AASS is a bifunctional enzyme with an N-terminal lysine-2-oxoglutarate reductase (LOR) domain and a C-terminal saccharopine dehydrogenase (SDH) domain, which are homologous to Saccharomyces cerevisiae LYS1 and LYS9, respectively. The LOR domain catalyses the reductive deamination of L-lysine and 2-oxoglutarate into saccharopine (EC 1.5.1.8), which constitutes the first committed, and possibly rate-limiting, step in lysine degradation. The LOR domain itself consists of two lobes, both Rossman folds with a central beta-sheet with alpha helices on the outside. Moreover, AASS is a unique drug target for inborn errors of metabolism such as glutaric aciduria type 1 that arise from deficiencies downstream in the lysine degradation pathway.

Remarkably, NEM potently activated LOR activity. The activation was not only concentration-dependent but also time-dependent, consistent with a covalent modification. Alkylation of LOR by NEM paralleled the activation pattern. Using X-ray crystallography (see below), we identified Cys 414 as alkylated by NEM. In the structure, there was unambiguous electron density for alkylation at only one position, Cys 414. We were able to model the NEM, which becomes N-ethylsuccinimide upon reaction with the cysteine, in the density and refine it with restraints for the sulfur-carbon bond. Interestingly, there are no obvious other differences between the apo and NEM structures. However, Cys 414 sits at the interface of the two lobes of the LOR, suggesting it is an important location for regulating activity. Subsequently, we were able to identify biochemically that Cys 414 is a key residue in the activation of LOR. We provide evidence that AASS can be activated in vitro by alkylation of Cys 414 using NEM. This modification suggests a novel site of allosteric activation of the enzyme, although the mechanism is still unknown.

>[4x]GSHHKAVLAVRREDVNAWERRAPLAPKHIKGITNLGYKVLIQPSNRRAIHDKDYVKAGGILQEDISEACLILGVKRPPEEKLMSRKTYAFFSHTIKAQEANMGLLDEILKQEIRLIDYEKMVDHRGVRVVAFGQWAGVAGMINILHGMGLRLLALGHHTPFMHIGMAHNYRNSSQAVQAVRDAGYEISLGLMPKSIGPLTFVFTGTGNVSKGAQAIFNELPCEYVEPHELKEVSQTGDLRKVYGTVLSRHHHLVRKTDAVYDPAEYDKHPERYISRFNTDIAPYTTCLINGIYWEQNTPRLLTRQDAQSLLAPGKFSPAGVEGCPALPHKLVAICDISADTGGSIEFMTECTTIEHPFCMYDADQHIIHDSVEGSGILMCSIDNLPAQLPIEATECFGDMLYPYVEEMILSDATQPLESQNFSPVVRDAVITSN>[2x]AAMADPYFECSMNTAVSFSGIIFYEQSHEYLDAEPGDPEGPNGEIYPARRF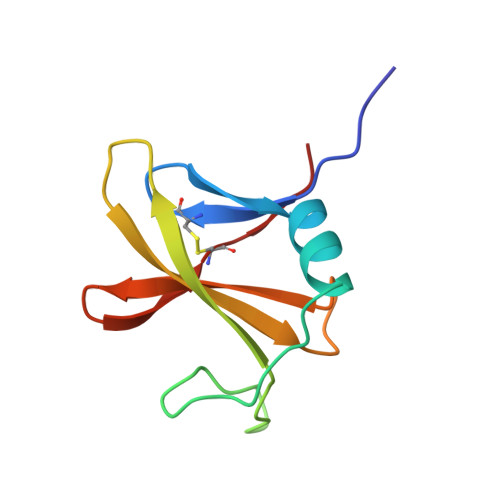TRVRRDGSDVLILIQSLDEYPLRRAYEKTEQGWRLCPFHKP(6~{R})-5,5-dimethyl-7-thia-2-azatricyclo[6.3.1.0^{4,12}]dodeca-1(12),3,8,10-tetraene-6-carboxylic acid | C13 H13 N O2 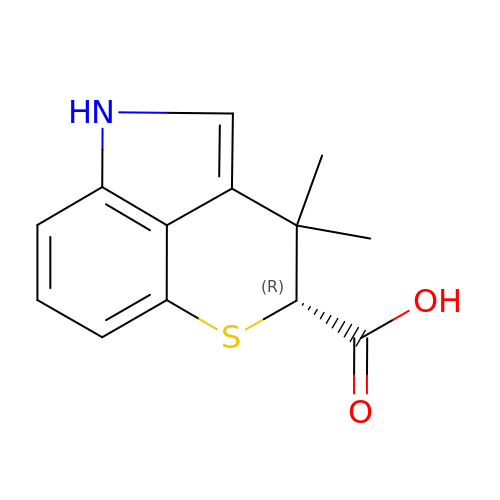S | PAGACRNFPGTTHG-NSHDSACASA-N>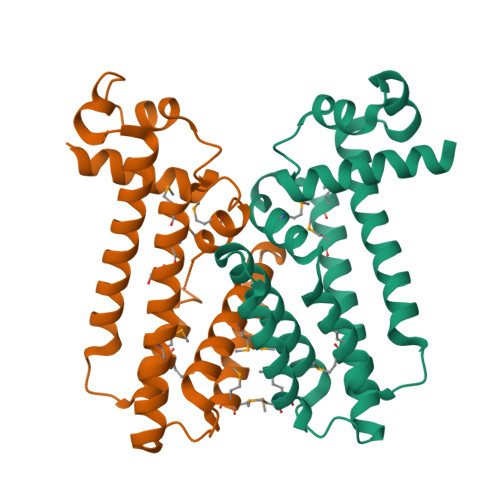[2x]SNAMTTHQVKKSEAKRQHILDSGFHLVLRKGFVGVGLQEILKTSGVPKGSFYHYFESKEAFGCELLKHYISDYQIRLNQLWTTETSARDKLMNYLQCWVKDPATEQSWAESCLIVKMAAEVADLSEDMRLIMNDGVKRLIARMADLIRIGQQEGSIQTSVVPDVLAQVIYQMYLGAALLSKLYKHKAPLFQALESTKMMLDGCNHVQQDKNQ>QVTVQSSPNFTQHVREQSLVTDQLSRRLIRTYQLYSRTSGKHVQVLANKRINAMAEDGDPFAKLIVETDTFGSRVRVRGAETG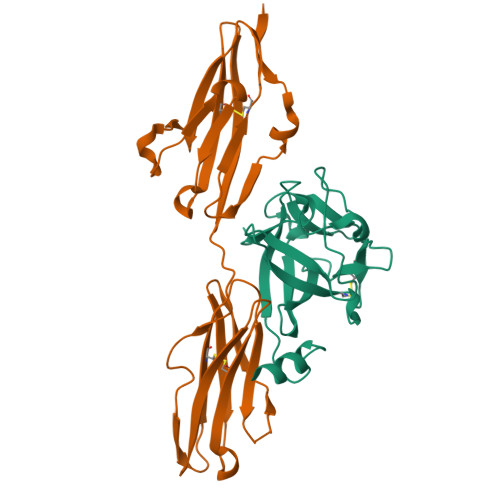LYICMNKKGKLIAKSNGKGKDCVFTEIVLENNYTALQNAKYEGWYMAFTRKGRPRKGSKTRQHQREVHFMKRLPRGHHTTE[2x];>[2x]NNKRAPYWTNTEKMEKRLHAVPAANTVKFRCPAGGNPMPTMRWLKNGKEFKQEHRIGGYKVRNQHWSLIMESVVPSDKGNYTCVVENEYGSINHTYHLDVVERSRHRPILQAGLPANASTVVGGDVEFVCKVYSDAQPHIQWIKHVEKNGSKYGPDGLPYLKVLKAAGVNTTDKEIEVLYIRNVTFEDAGEYTCLAGNSIGISFHSAWLTVLPAPGREKE(2S)-2-{2-[(4-chloro-2-methylphenoxy)methyl]-6-fluoro-1H-benzimidazol-1-yl}-N,2-dicyclohexylacetamide | C29 H35 Cl F N3 O2 | 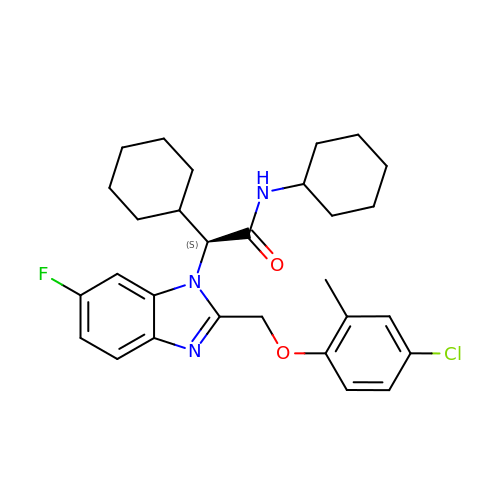MAXDJYGVHNACQO-NDEPHWFRSA-N> HXEGXFTSDLSKQMEEEAVRLFIEWLK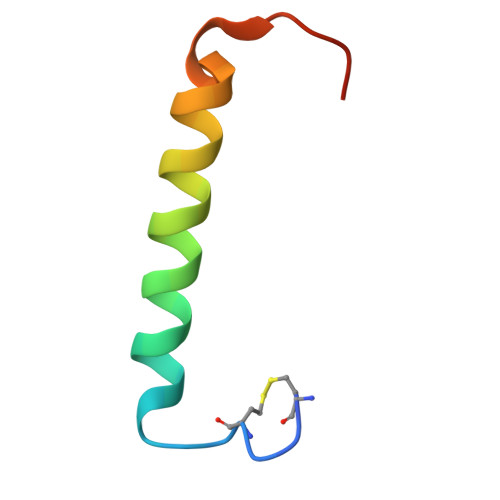NGGPSSGAPPPS>MSEIITFPQQTVVYPEINVKTLSQAVKNIWRLSHQQKSGIEIIQEKTLRISLYSRDLDEAARASVPQLQTVLRQLPPQDYFLTLTEIDTELEDPELDDETRNTLLEARSEHIRNLKKDVKGVIRSLRKEANLMASRIADVSNVVILERLESSLKEEQERKAEIQADIAQQEKNKAKLVVDRNKIIESQDVIRQYNLADMFKDYIPNISDLDKLDLANPKKELIKQAIKQGVEIAKKILGNISKGLKYIELADARAKLDERINQINKDCDDLKIQLKGVEQRIAGIEDVHQIDKERTTLLLQAAKLEQAWNIFAKQLQNTIDGKIDQQDLTKIIHKQLDFLDDLALQYHSMLLS[4x]

We have unraveled structures of the soluble components and the pore assembly of the YaxAB cytolysin from Y. enterocolitica. The crystal structures show an atypical fold, comprising a head domain reminiscent of ClyA family toxins and pronounced coiled-coil and foot domains unique to the YaxAB system. In line with our finding that the isolated YaxA and YaxB head domains form spoked oligomers in solution, the YaxB head domain in isolation was sufficient for recruitment to membrane-bound YaxA. Together, our biochemical data support a role for YaxA as the initial membrane-interacting subunit of the toxin, able to bring the lytic effector YaxB to the target cell surface. Therefore, we propose that this class of toxins defines a new structural family of α-PFTs.

The orthologue PaxB produced better diffracting crystals than YaxB and thus served as template for molecular replacement phasing (the two proteins share 40% amino acid sequence identity, whereas YaxA shares 18% and 22% sequence identity with PaxB and YaxB, respectively). YaxA and PaxB crystal structures were determined using single-wavelength anomalous dispersion (SAD) on selenomethionine-derivatized proteins. Because our PaxB model could be well resolved, missing merely the N-terminal 11 residues, we will utilize these coordinates for most structural analyses throughout the manuscript. All three proteins adopt similarly elongated, α-helical folds composed of a five-helix bundle head domain and a two-helix-coiled-coil stalk, tapering to a narrow turn in the case of YaxA, while connecting to an additional α-helical domain in the case of PaxB. For the PaxB head domain, Z-scores ranged from 7.4 (soluble-monomeric ClyA, 3.8 Å RMSD) to 13.3 (pore-protomeric ClyA, 2.4 Å RMSD; PDB code 2WCD12). Our monomeric PaxB structure, while complete, might hamper a true comparison with the protomeric YaxB unit, since it is derived from a different species. However, it is noteworthy that the foot domain represents the region of highest sequence conservation between Yersinia and Photorhabdus orthologues (60% sequence identity; Supplementary Figure 12b, highlighted in black box), indeed pointing to a common principle of pore formation.>DTNVKQVKVLQLINAYRFRGHQHANLDPLGLYQQDKVADLDPSFHDLTEADFQETFNVGSFASGKETMKLGELLEALKQTYCGPIGAEYMHITSTEEKRWIQQRIESGRATFNSEEKKRFLSELTAAEGLERYLGAKFPGAKRFSLEGDALIPMLKEMIRHAGNSGTREVVLGMAHRGRLNVLVNVLGKKPQDLFDEFAGKHKEHLGTGDVKYHMGFSSDFQTDGGLVHLALAFNPSHLEIVSPVVIGSVRARLDRLDEPSSNKVLPITIHGDAAVTGQGVVQETLNMSKARGYEVGGTVRIVINNQVGFTTSNPLDARSTPYMTDIGKMVQAPIFHVNADDPEAVAFVTRLALDFRNTFKRDVFIDLVCYRRHGHNEADEPSATQKIKKHPTPRKIYADKLEQEKVATLEDATEMVNLYRDALDAGDCVVAEWRPMNMHSFTWSPYLNHEWDEEYPNKVEMKRLQELAKRISTVPEAVEMQSRVAKIYGDRQAMAAGEKLFDWGGAENLAYATLVDEGIPVRL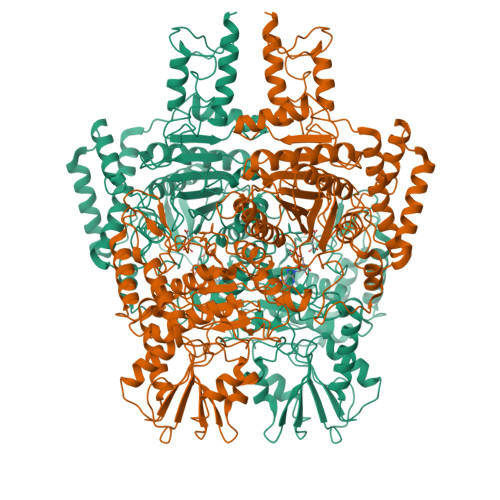SGEDSGRGTFFHRHAVIHNQSNGSTYTPLQHIHNGQGAFRVWDSVLSEEAVLAFEYGYATAEPRTLTIWEAQFGDFANGAQVVIDQFISSGEQKWGRMCGLVMLLPHGYEGQGPEHSSARLERYLQLCAEQNMQVCVPSTPAQVYHMLRRQALRGMRRPLVVMSPKSLLRHPLAVSSLEELANGTFLPAIGEIDELDPKGVKRVVMCSGKVYYDLLEQRRKNNQHDVAIVRIEQLYPFPHKAMQEVLQQFAHVKDFVWCQEEPLNQGAWYCSQHHFREVIPFGASLRYAGRPASASPAVGHMSVHQKQQQDLVNDALNVE[2x]N-myristoyltransferase (NMT) is a promising antimalarial drug target. NMT cotranslationally transfers the myristate moiety of myristoyl-coenzyme A (MyrCoA) to Gly2 of protein substrates after removal of the N-terminal methionine.17−19P. vivax and P. falciparum express a single NMT protein, whereas human cells express two closely related isotypes, HsNMT1 and HsNMT2.20PvNMT and PfNMT have more than 80% shared identity, while the human orthologs are only about 40% identical in sequence to PvNMT and PfNMT. Small-molecule inhibitors bind both PvNMT and HsNMT1 in the peptide binding cleft, where residues contacting the ligands via side chain atoms share 100% sequence identity. The inhibitor binding site is located within the peptide binding cleft formed by the N- and C-terminal domains.

Strikingly, however, replacing the morpholine with acetate caused an increase in selectivity for a pyridine core (9c) and a sharp decrease for a phenyl core (8c). The electron density, however, is weak for the tail group extension of 9c and indicates multiple conformations. Two copies of 9c were built into each active site. However, the tail group and extension of 9c are unstably bound, with six conformations modeled. Of these, two consistent conformers (observed in more than one chain) have the amide carbonyl directed either toward the side chain of Asn365 or that of Ser319. The carboxylate does not appear to form hydrogen bonds with the protein. In the presence of the 9c dynamics, the His213 side chain adopts both inwardly and outwardly pointing rotamers (A and B, respectively), but considering all three asymmetric unit copies, samples the B state with higher occupancy. The pyridine of 9c draws a water molecule closer through hydrogen bonding thereby enabling the incorporation of an extra water. Within the complex with 9c, the N4 ammonium interacts electrostatically with the side chains of Asn161 and Thr197 and the carboxylate of Leu410 but is situated in closer proximity to the side chains.

>[3x]GPDYKFWYTQPVPKINDEFNESVNEPFISDNKVEDVRKDEYKLPPGYSWYVCDVKDEKDRSEIYTLLTDNYVEDDDNIFRFNYSAEFLLWALTSPNYLKTWHIGVKYDASNKLIGFISAIPTDICIHKRTIKMAEVNFLCVHKTLRSKRLAPVLIKEITRRINLENIWQAIYTAGVYLPKPVSDARYYHRSINVKKLIEIGFSSLNSRLTMSRAIKLYRVEDTLNIKNMRLMKKKDVEGVHKLLGSYLEQFNLYAVFTKEEIAHWFLPIENVIYTYVNEENGKIKDMISFYSLPSQILGNDKYSTLNAAYSFYNVTTTATFKQLMQDAILLAKRNNFDVFNALEVMQNKSVFEDLKFGEGDGSLKYYLYNWKCASFAPAHVGIVLL(2S)-2-[3-(AMINOMETHYL)PHENYL]-3-[(R)-HYDROXY{(1R)-2-METHYL-1-[(PHENYLSULFONYL)AMINO]PROPYL}PHOSPHORYL]PROPANOIC ACID | C20 H27 N2 O6 P S | 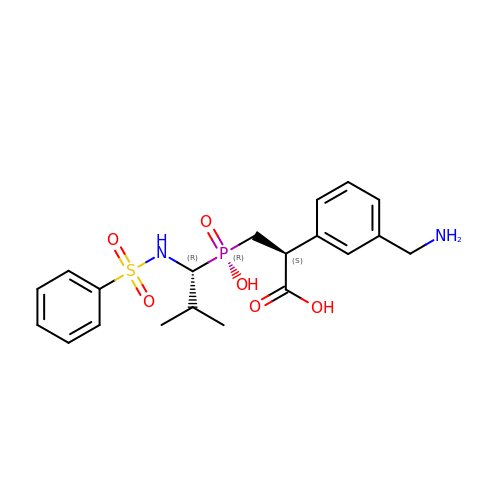FNZHLCNFXRRIIC-RBUKOAKNSA-N> GPGSEFVRRVKTIYDCQADNDDELTFIEGEVIIVTGEEDQEWWIGHIEGQ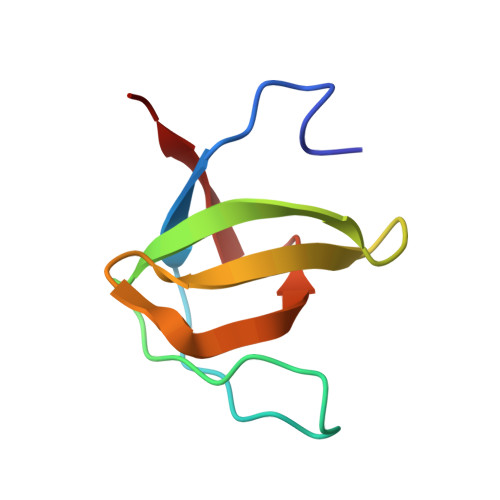PERKGVFPVSFVHILSD> GSKKIDDDLFEELEEQLLIADVGVE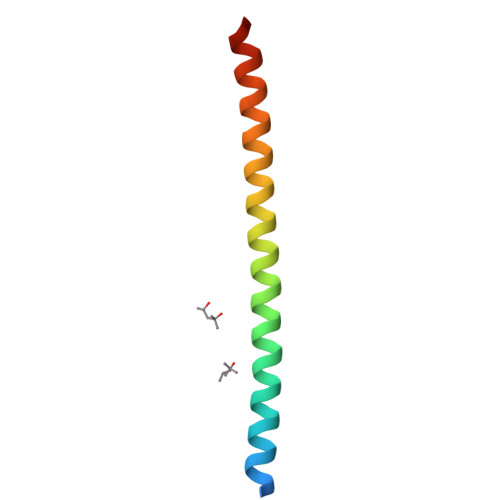TTRKIITNLTEGASRKQLRDAEALYGLLKEEMGEILA>[2x]VPGTLLPRLPSEPGMTLLTIRIEKIGLKDAGQCIDPYITVSVKDLNGID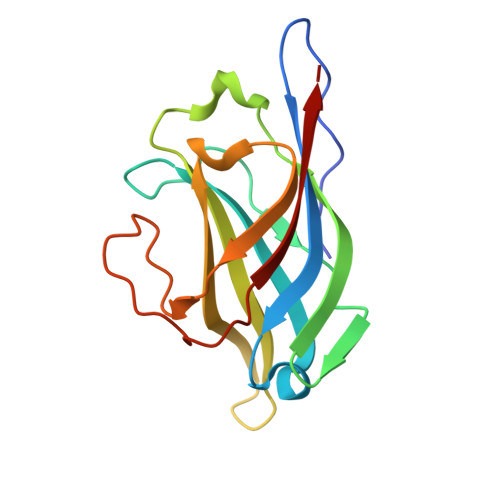LTPVQDTPVASRKEDTYVHFNVDIELQKHVEKLTKGAAIFFEFKHYKPKKRFTSTKCFAFMEMDEIKPGPIVIELYKKPTDFKRKKLQLLTKKPLYLHLHQSLHKE> SQAGDTLNDVIQDPTRRNKLINDNNLLKGIIMGRDGPVPSSRELIVRPDTLRAIINNRATIETTTMEAEFTETLMESNYNSASVKVSAPFITANSEYSESSSFKNTETEKSMYTSSRYLFPQGRIDFTTPDSGFDDVIKLSPQFTSGVQAALAKATGTEKREALQNLFQEYGHVFRTKVHIGGVLSAHTMETFSRSENETEVKQDVKAGLEGAVKGWGGGATAGHGNTQGTITTSQNRKLNVKYIVNGGDYTKIQNTEEWVASTNQSEHWRVIEVTEVTAVADLLPQPIRGQVKDLLKPLLGKWVDVEKVPGLESLPVSVYRPKGAIP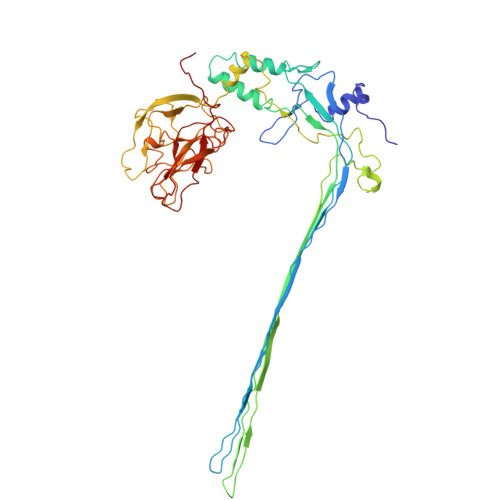AGWFWLGDTADASKALLVKPTLPARSGRNPALTSLHQGSGMTEQPFVDLPQYQYLSTYFGSFAHDTPPGSTLRGLRPDHVLPGRYEMHGDTISTAVYVTRPVDVPFPEDECFDLKSLVRVKLPGSGNPPKPRSALKKSMVLFDSGEK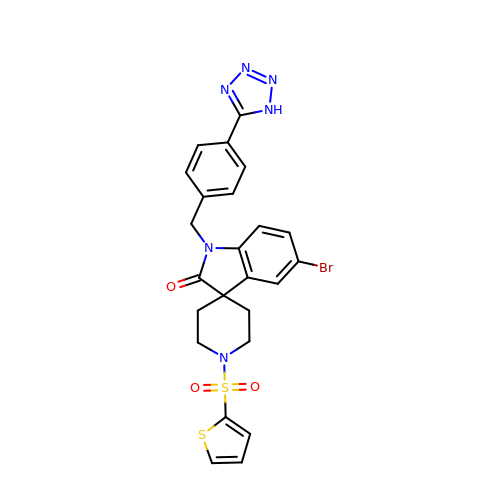5-bromo-1-{[4-(1H-tetrazol-5-yl)phenyl]methyl}-1'-(thiophene-2-sulfonyl)spiro[indole-3,4'-piperidin]-2(1H)-one | C24 H21 Br N6 O3 S2 | PDMCUTCDLHMYSW-UHFFFAOYSA-N>[6x]KTVNLSACEVAVLDLYEQSNIR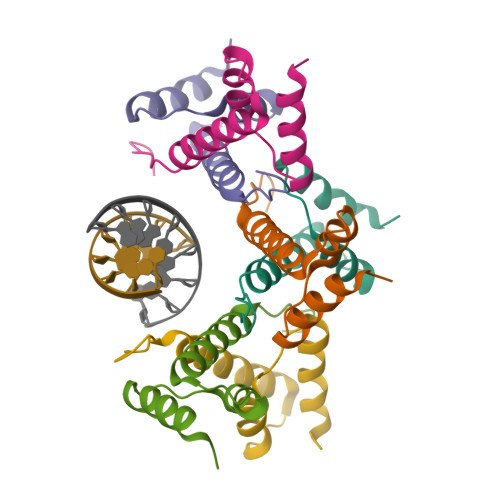IPSDIIEDLVNQRLQSEQEVLNYIETQRTYWKLENQKKLYRGSLK> AHHHHHHGSNSKEFRKIALVGASKNPAKYGNIILKDLLSKGFEVLPVNPNYDEIEGLKCYRS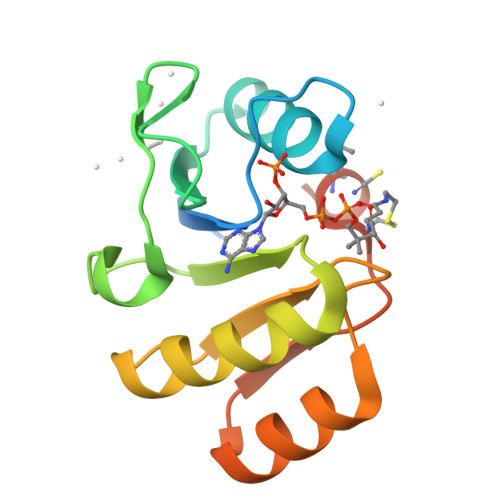VRELPKDVDVIVFVVPPKVGLQVAKEAVEAGFKKLWFQPGAESEEIRRFLEKAGVEYSFGRCIMVETSNKKIFLEV>GSMTSSGSSRDLFRALNSFIQTPTLPPPADLDAIISSYLERHDKPEEGSGDRLNDELLAIWDKAVQDHPEKYAAFVAVLRQLRPGLGAPARTFQWWDKLLDPVLDNATREKGLARSFMDFTLEILSSSEYDDPEAWGEEGFIPWLNRLLVRWMELRESRADFRPSTDLKEQVLTDALLAFGKKDPKGFMNALNAFVLRREHRNSAFSLLCAFVNSGPPHLYLILQTPLFGNILQSLQKDESTFTVNLALIALVMLLPFFPGDIVPYLPTLFNIYARLLFWDRDSYFAQQHTEMGENHGESGTDTPWDKVLLDPDYDG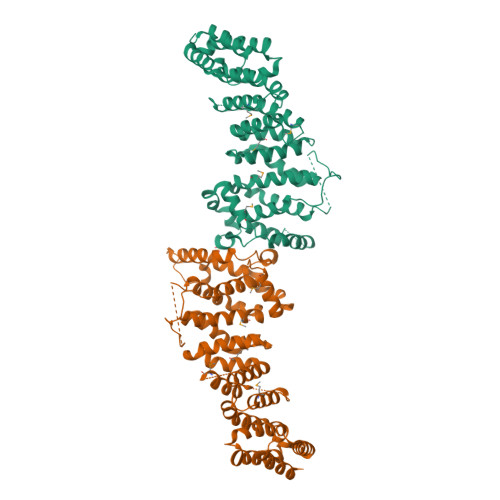HSVPYLPEYFTILYGLYPINFVDYIRKPHNYLPHAGSDDDIDVHAAEIRERSERFRKQHLLHPNFYEYTIETEKTNITRWLKSEADEIIADCMALVVDRG[4x]>MQLLSGIVQQRNNMLRAIEAQQHLLQLTVWGIKQLQARILAGGRGGHTTWMEWDREINNYTSLIHSLIEESQNQQ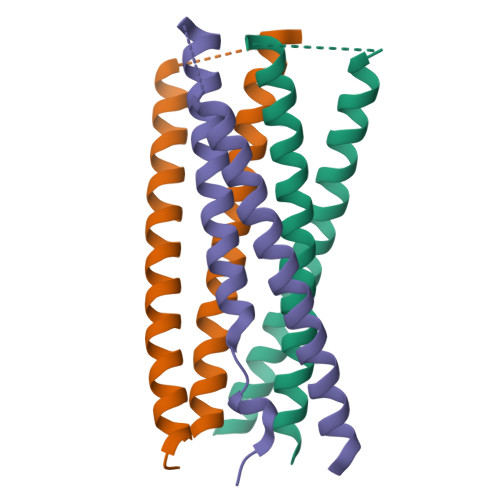EKNEQELLGGHHHHHH[3x]> MRINSELANKFSASTVHLEHITTALSCLTPFGSKDDVLIFIDADGLSFVRENNHVIKIQLLLSRELFMSYSYRNETEDHMKLCVKINHILDSVSVMNRNSDDIVECTLSYDGHGSPFVLIFEDSFISERVEYSTYLIKDFDTNGLELDRERISFEAIIKGEALHSALKDLKEIGCKECYVYAKTEANDENVFALISKSQLGFSKIKLPSNRSILEKLQVFDGDSTTVIDGFAVIGFFDFTSFDKIRKSTKIASKVLFRMDVHGVLSVNILSQTDDVIITDTTRPSNNRPGSIRQLQLPKDYPGIVIEVCMLEKESIDEAAQTEIELLMETNELGNRNSFKKSTIRKRYGTDKGNETSNDNLLQLNGKKIKLPSEEENNKNRESED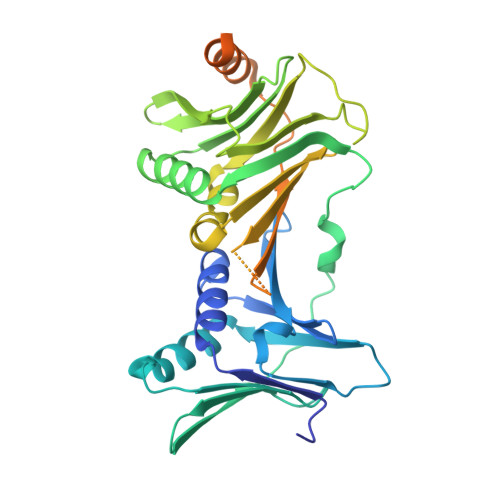EENHCKYPTKDIPIFF>[2x]GSHMVRESSFVEKMKKTGRNIIVFYGSQTGTAEEFANRLSKDAHRYGMRGMSADPEEYDLADLSSLPEIDNALVVFCMATYGEGDPTDNAQDFYDWLQETDVDLSGVKFAVFGLGNKTYEHFNAMGKYVDKRLEQLGAQRIFELGLGDDDGNLEEDFITWREQFWLAVCEHFGVEATGEESSIRQYELVVHTDIDAAKVYMGEMGRLK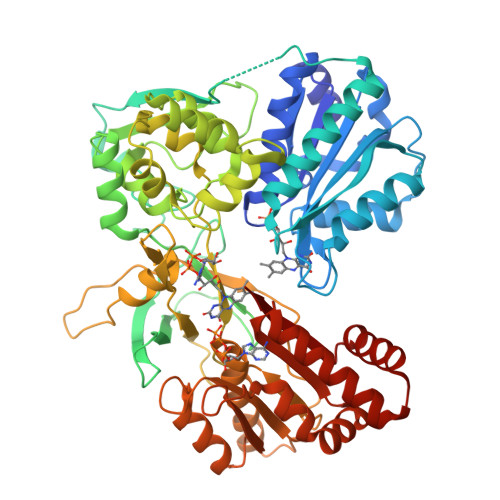SYENQKPPFDAKNPFLPAVTTNRKLNQGTERHLMHLELDISDSKIRYESGDHVAVYPANDSALVNQLGKILGADLDVVMSLNNLDEESNKKHPFPCPTSYRTALTYYLDITNPPRTNVLYELAQYASEPSEQELLRKMASSSGEGKELYLSWVVEARRHILAILQDCPSLRPPIDHLCELLPRLQARYYSIASSSKVHPNSVHICAVVVEYETKAGRINKGVATNWLRAKEPVGENGGRALVPMFVRKSQFRLPFKATTPVIMVGPGTGVAPFIGFIQERAWLRQQGKEVGETLLYYGCRRSDEDYLYREELAQFHRDGALTQLNVAFSREQSHKVYVQHLLKQDREHLWKLIEGGAHIYVCGDARNMARDVQNTFYDIVAELGAMEHAQAVDYIKKLMTKGRYSLDVWS>SNAMLRRLFKKKYVCVRQYDLTDCGAACLSSIAQYYGLKMSLAKIREMTGTDTQGTNAYGLIHAAKQLGFSAKGVKASKEDLLKDFRLPAIANVIVDNRLAHFVVIYSIKNRIITVADPGKGIVRYSMDDFCSIWTGGLVLLEPGEAFQKGDYTQNMMVKFAGFLKPLKKTVLCIFLASLLYTALGIAGSFYIKFLFDDLIKFEKLNDLHIISAGFAVIFLLQIFLNYYRSILVTKLGMSIDKSIMMEYYSHVLKLPMNFFNSRKVGEIISRFMDASKIRQAISGATLTIMIDTIMAVIGGILLYIQNSSLFFISFIIILLYGIIVTVFNKPIQNANRQIMEDNAKLTSALVESVKGIETIKSFGAEEQTEKSTRDKIETVMKSSFKEGMLYINLSSLTGIVAGLGGIVILWAGAYNVIKGNMSGGQLLAFNALLAYFLTPVKNLIDLQPLIQTAVVASNRLGEILELATEKELREDSDDFVISLKGDIEFRNVDFRYGLRKPVLKNINLTIPKGKTVAIVGESGSGKTTLAKLLMNFYSPEKGDILINGHSIKNISLELIRKKIAFVSQDVFIFSGTVKENLCLGNENVDMDEIIKAAKMANAHDFIEKLPLKYDTFLNESGANLSEGQKQRLAIARALLKKPDILILDEATSNLDSITENHIKDAIYGLEDDVTVIIIAHRLSTIVNCDKIYLLKDGEIVESGSHTELIALKGCYFKMWKQTENTLAS[2x]

Peptidase-containing ABC transporters (PCATs) in gram-positive bacteria function both as maturation proteases and exporters for biofilm formation, quorum sensing, or antimicrobial polypeptides. Substrates of PCATs are synthesized as precursors with an N-terminal leader peptide. Proteolytic cleavage of the leader peptide at the conserved double-glycine motif is necessary for secretion of the cargo peptide. In this work, we determined the structures of wild-type PCAT1 (wtPCAT1) in the presence of substrate and ATP with or without Mg2+.

To obtain a structural basis for this biochemical property, wtPCAT1 was vitrified in the presence of excess substrate and ATP. Mg2+ ion was omitted to prevent ATP hydrolysis. Cryo-EM reconstruction resulted in a predominant conformation at an overall resolution of 4.5 Å. Density modification further improved the map, showing side chain densities for the dimerized NBDs as well as ligand densities that are consistent with ATP. In the presence of ATP without Mg2+, wtPCAT1 adopts an outward-facing (OF) conformation in which the NBDs form a closed dimer, and the translocation pathway opens to the extracellular space. The intracellular, lateral opening of the translocation pathway observed in the IF conformations is completely closed. The PEP domains are flexibly attached to the core transporter, with no defined interactions with the TMDs or the NBDs. No density corresponding to the substrate is observed, possibly due to the limited resolution of the PEP domains. In the absence of Mg2+, PCAT1 predominately exhibits an OF conformation, in which the PEP domains are detached from the translocation pathway, the NBDs are dimerized with two ATP molecules poised for hydrolysis, and the cargo substrate has been released. Using Eq. 2, we conclude that the energy of the OF conformation is lower than that of the IF conformation.4-{[4-(acetylamino)-1-methyl-1H-pyrrole-2-carbonyl]amino}-1-methyl-N-{4-[(1-methyl-1H-pyrrol-3-yl)amino]-4-oxobutyl}-1H-imidazole-2-carboxamide 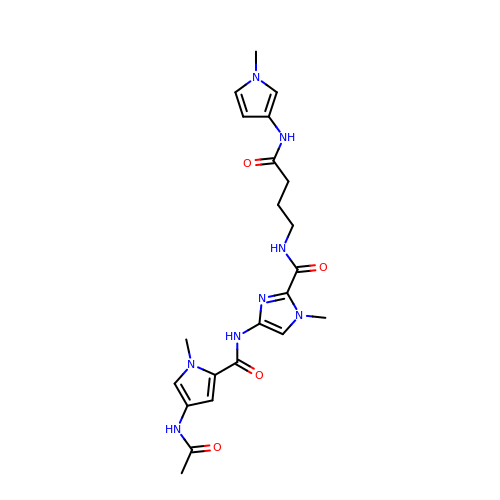| C22 H28 N8 O4 | LQGDWGRHWDPWIC-UHFFFAOYSA-N>[3x]GSLDDSISAASTSDVQDRLSALESRVQQQEDEMTVLKAALADVLRRLAISEDHVA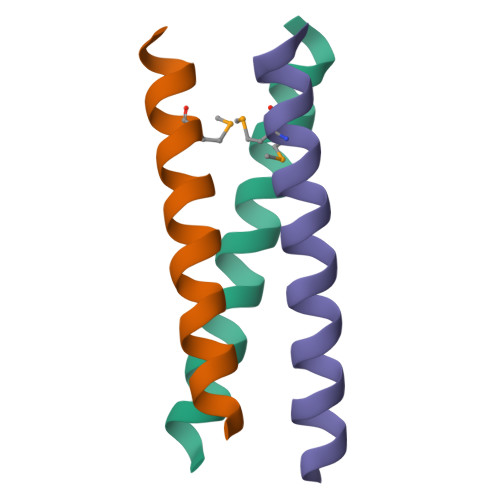SVKK>SYDDTRQHLLDTGYRIMAVKGFSGVGLNEILQSAGVPKGSFYHYFKSKEQFGQALLEDYFRVYLADMDQRFSAPGLNARERLMSYWQKWLDNACPPCDEQRCLVVKLSAEVADLSESMRITLRDGSDGIIERLVGCLGQGRDDGSLAPCDARHMASALYQLW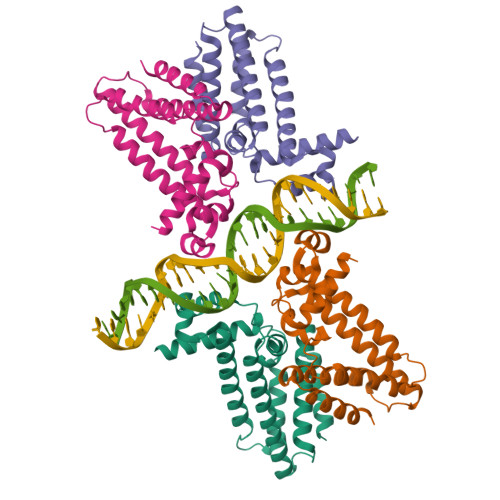LGASLLSKLHRSPGPLETAMQTTRSLLE[16x]>[8x]M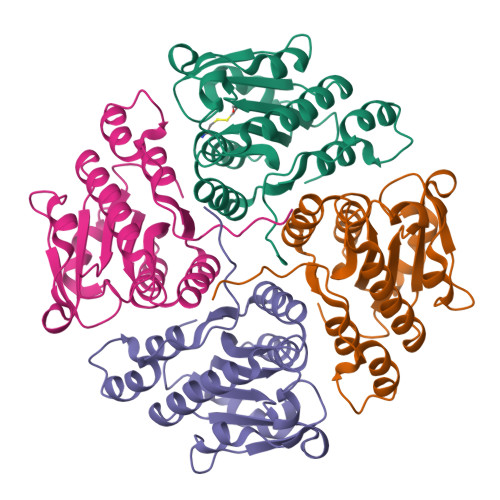AARKLIARINPTNSALFVCDLQEKFASNIKYFPEIITTSRRLIDAARILSIPTIVTEQYPKGLGHTVPTLKEGLAENTPIFDKTKFSMCIPPTEDTLKKVQNVILVGIEAHVCVLQTTYDLLERGLNVHVVVDAVSSRSHTDRHFAFKQMEQAGAILTTSEATILGLVGGSDHPKFKEVQKLILTSAPDTGLVPLSKL> KTRTKVYYQEIQKEENAK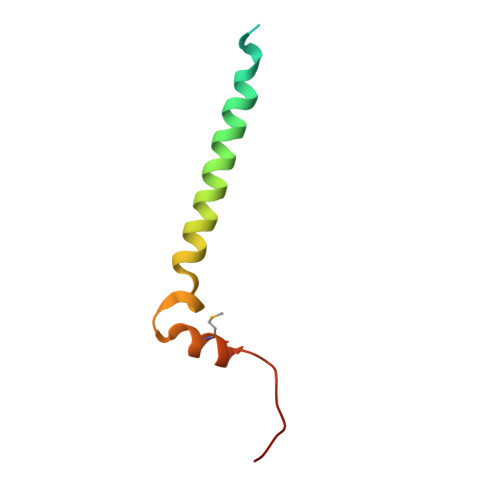AKEIAQQEKLQEDKDAKDKREKELLVAQFRRLGGLERMVGELDIKFDLKF naphthalene-1,3-diol 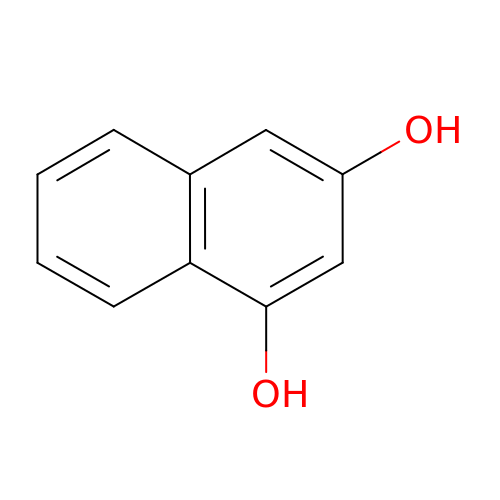| C10 H8 O2 | XOOMNEFVDUTJPP-UHFFFAOYSA-N>MYKWSTEVGEIIIARNRDGHFYINAFVNNVKIKFMVDTGASDIALTKEDAQKLGFDLTKLKYTRTYLTANGENKAAPITLNSVVIGKE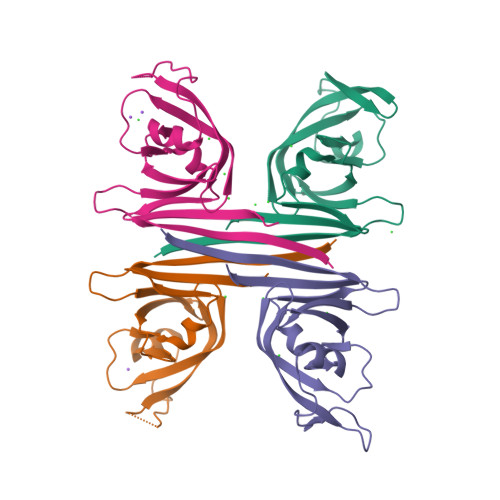FKNIKGHVGLGDLDISLLGMSLLERFKGFRIDKDLLILNYAAALEHHHHHH[4x]> GPLGSWVIPPISCPENEKGPFPKNLVQIKSNKDKEGKVFYSITGQG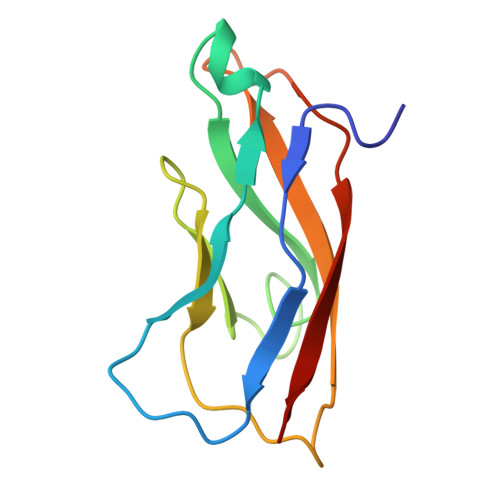ADTPPVGVFIIERETGWLKVTEPLDRERIATYTLFSHAVSSNGNAVEDPMEILITVTDQ> MARDEVRRILPADIKREVLIKDENAETNPDWGFPPEKRPIEMHIQFGVINLDK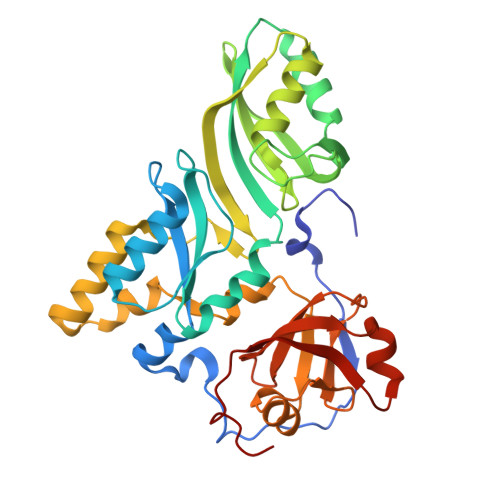PPGPTSHEVVAWIKKILNLEKAGHGGTLDPKVSGVLPVALEKATRVVQALLPAGKEYVALMHLHGDVPEDKIIQVMKEFEGEIIQRPPLRSAVKRRLRTRKVYYIEVLEIEGRDVLFRVGVEAGTYIRSLIHHIGLALGVGAHMSELRRTRSGPFKEDETLITLHDLVDYYYFWKEDGIEEYFRKAIQPMEKAVEHLPKVWIKDSAVAAVTHGADLAVPGIAKLHAGIKRGDLVAIMTLKDELVALGKAMMTSQEMLEKTKGIAVDVEKVFMPRDWYPKL CT and LT, with their five equivalent binding subunits, are known to be multivalent proteins. Binding has been described as a “two-fingered grip”, provided by the two terminal residues, galactose (Gal) and sialic acid (NeuAc). The specificity of this interaction is mainly determined by the terminal galactose residue, which is buried in a deep pocket at the rugged underside of the toxin (distant from the A-subunit). As expected, all three inhibitors bind in the primary binding site, acting as decoys for the toxins’ main receptor, the GM1 ganglioside.

Compounds 2 and 3 are bidentate ligands that combine the two terminal residues of the GM1 oligosaccharide, i.e. galactose and sialic acid. The cholera toxins come in two varieties: classical (c) and El Tor (ET). The two biotypes differ at two amino acid residues in the B-subunit, 18 and 47 (His18 and Thr47 in cCTB, and Tyr18 and Ile47 in ET CTB). The crystal structures were solved to 1.1 Å resolution and contain one B-pentamer in the asymmetric unit. Both CT variants have well-defined electron density for inhibitor 2 in all binding sites. As in the other structures, the galactose moiety of 2 is buried in the GM1 binding site, H-bonding with Glu51, Gln61, Asn90 and Lys91. The sialic acid residue has direct interactions with the backbones of Glu11 and His13. The differences to GM1-os binding can be seen in the linker region of 2, where the hydrogen bond of the core Gal to the side chain of His13 is no longer achievable. Instead, closer to the terminal Gal, the carbonyl group of the linker engages in a water-mediated interaction to Asn14.

>[5x]TPQNITDLCAEYHNTQIYTLNDKIFSYTESLAGKREMAIITFKNGAIFQVEVPGSQHIDSQKKAIERMKDTLRIAYLTEAKVEKLCVWNNKTPHAIAAISMAN> GSMASSSTAYYLKDAGFHIRNIPKAWNDWNLFHVFQNFGKVSYCRVVGQSNDGQVQLGFVNMMSVADADEVRKNMNDGNLIGENFTLKV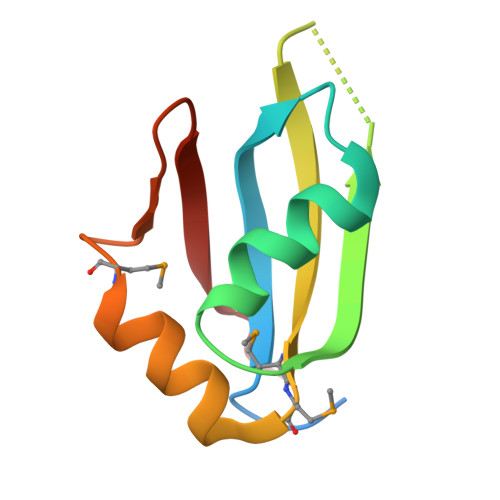TDHKN>MKYQLSATEARVIGCLLEKQVTTPEQYPLSVNAVTMACNQKTNREPVMNLGE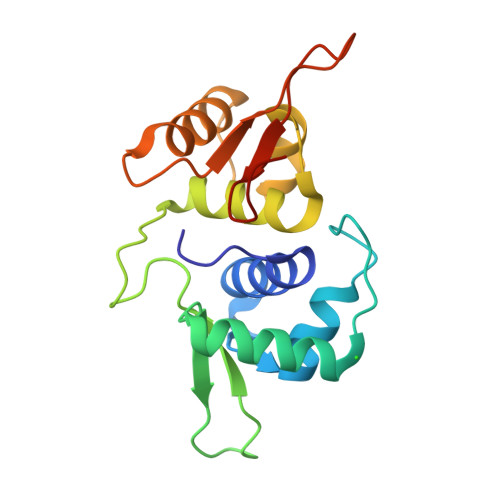HEVQDILDELVKRHYLRTVSGFGNRVTKYEQRFCNSEFGDLKLSAAEVAVITTLLLRGAQTPGELRTRASRMHEFADMQEVEQTLDGLATREDGPYVVRLAREPGKRESRYMHLFSGEVDTST[4x]>SITSDDSLEVIARKLNREKELALEQTCALLDYARLQKIIEVISKAPFIQITGLGGSALVGRDLSFKLMKIGYRVACEADTHVQATVSQALKKGDVQIAISYSGSKKEIVLCAEAARKQGATVIAITSLTDSPLRRLAHFTLDT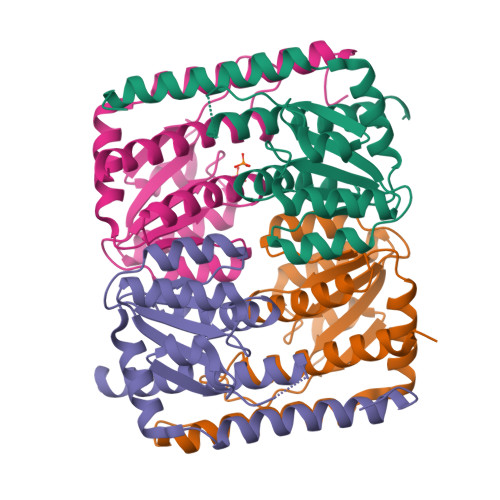VSGETEWRSSSMSTRTAQNSVTDLLFVGLVQLNDVESL[4x]>[4x]DAQIIIPNGNY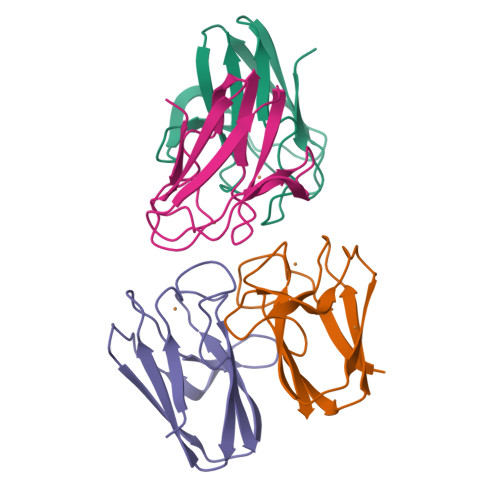DVTGAGFYSPLNLEIPVGTTVTWTNDDSVPHNIQSIDVNGKVIQLFNSPPLNTGDRFEHVFEEEGVYKYYCSFHPWRVGLVTVS> RLLEDALIAVRQQTAMMRKFLDTPGKLMDALKCCSTLV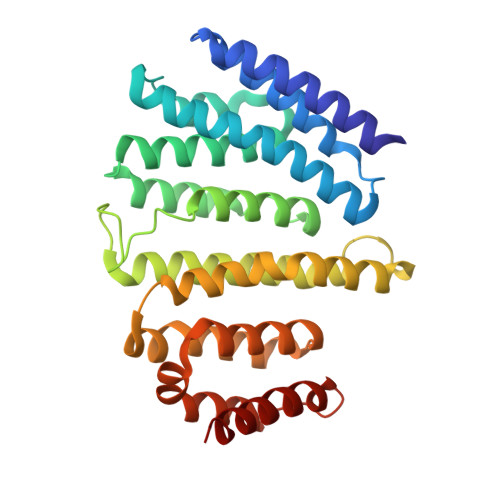SELRTSSLSPKQYYELYMAVFDALRYLSAHLRENHPVNHLADLYELVQYAGNIIPRLYLMITVGTAYMSIDGAPVKELMKDMMDMSRGVQHPVRGLFLRYYLSGQARDYLPTGDSDGPEGNLQDSINFILTNFVEMNKLWVRLQHQGHSRERDLRTQERRELQLLVGSNIVRLSQLVDLPTYRDSILGPLLEQIVQCRDILAQEYLLEVITQVFPDEYHLHTLDQFLGAVSRLNPHVNVKAIVIGMMNRLSDYAERE>[6x]GAMGSVANVGSHCDLSLKIPEISIQDMTAQVTSPSGKTHEAEIVEGENHTYCIRFVPAEMGTHTVSVKYKGQHVPGSPFQFTVGPLGEGGAHKVRAGGPGLERAEAGVP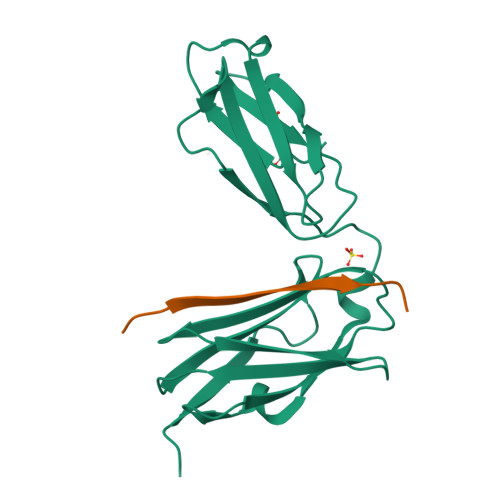AEFSIWTREAGAGGLAIAVEGPSKAEISFEDRKDGSCGVAYVVQEPGDYEVSVKFNEEHIPDSPFVVPVASPS;>PEKRVASSVFITLAPPRRDVAVAE[6x]>MAPEYWCSIAYFEMDVQVGETFK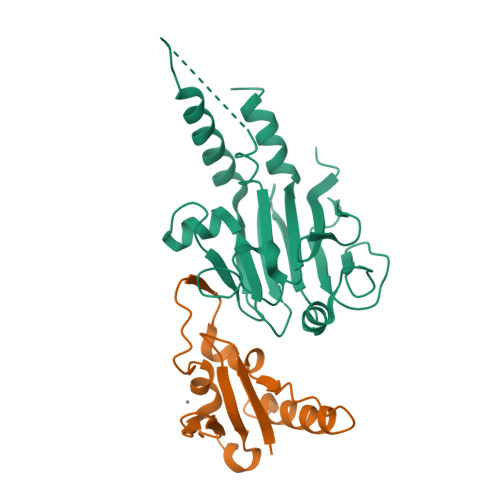VPSSCPIVTVDGYVDPSGGDRFCLGQLSNVHRTEAIERARLHIGKGVQLECKGEGDVWVRCLSDHAVFVQSYYLDREAGRAPGDAVHKIYPSAYIKVFDLRQCHRQMQQQAATAQAAAAAQAAAVAGNIPGPGSVGGIAPAISLSAAAGIGVDDLRRLCILRMSFVKGWGPDYPRQSIKETPCWIEIHLHRALQLLDEVLHTMPIADPQPLD[2x];>GSHMRVYHECFGKCKGLLVPELYSSPSAACIQCLDCRLMYPPHKFVVHSHKALENRTCHWGFDSANWRAYILLSQDYTGKEEQARLGRCLDDVKEKFDY[2x]> MLCSRYFTSSLFLWGEALPTLLEEFLNEVEKMLKNQVNTRRIHQLLKELDDPLLENKDLEEKLQAFLDYVKEIPNLPEARKRYRIQKSLEMIEKLRSWFLIDYLECSGEEVDLSTDIQYAKGVGPNRKKKLKKLGIETLRDLLEFFPRDYEDRRKIFKLNDLLPGEKVTTQGKIVSVETKKFQNMNILTAVLSDGLVHVPLKWFNQDYLQTYLKQLTGKEVFVTGTVKSNAYTGQYEIHNAEVTPKEGEYVRRILPIYRLTSGISQKQMRKIFEENIPSLCCSLKETLPERILEKRKLLGVKDAYYGMHFPKTFYHLEKARERLAYEELFVLQLAFQKIRKEREKHGGIPKKIEGKLAEEFIKSLPFKLTNAQKRAHQEIRNDMISEKPMNRLLQGDVGSGKTVVAQLAILDNYEAGFQTAFMVPTSILAIQHYRRTVESFSKFNIHVALLIGATTPSEKEKIKSGLRNGQIDVVIGTHALIQEDVHFKNLGLVIIDEQHRFGVKQREALMNKGKMVDTLVMSATPIPRSMALAFYGDLDVTVIDEMPPGRKEVQTMLVPMDRVNEVYEFVRQEVMRGGQAFIVYPLIEESDKLNVKSAVEMYEYLSKEVFPEFKLGLMHGRLSQEEKDRVMLEFAEGRYDILVSTTVIEVGIDVPRANVMVIENPERFGLAQLHQLRGRVGRGGQEAYCFLVVGDVGEEAMERLRFFTLNTDGFKIAEY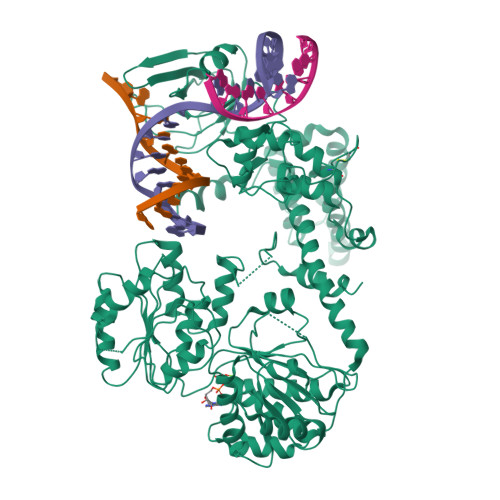DLKTRGPGEFFGVKQHGLSGFKVADLYRDLKLLEWAREDVQEIDVEGIELPEEIKLIEVG>MGSSHHHHHHSSGLRNAYTERDMLQKAADETTLKNVLVMKQAWVPYPAYTDRAAWDSLMGSNKQRLIAAGEKLLDYKWQLIPATAYLEYERTGNRKIMEVPYDANRQALNTLMLAELAEGKGRFIDQLLNGAYMSCEMNSWVLSAHLPRQSSKRSLPDFREQIIDLGSGGYGALMAWVHYFFRKPFDKINPVVSLQMRKAIKERILDPYMNDDDMWWMAFNWQPGEIINNWNPWCNSNALQCFLLMENNKDRLAKAVYRSMKSVDKFINFVKSDGACEEGTSYWGHAAGKLYDYLQILSDGTGGKISLLNEPMIRRMGEYMSRSYVGNGWVVNFADASAQGGGDPLLIYRFGKAVNSNEMMHFAAYLLNGRKPYATMGNDAFRSLQSLLCCNDLAKETPKHDMPDVTWYPETEFCYMKNKNGMFVAAKGGFNNESHNHNDVGTFSLYVNTIPVILDAGVGTYTKQTFGKDRYTIWTMQSNYHNLPMINGIPQKYGQEYKATNTTCNEKKRVFSTDIAAAYPSEAKVKNWIRSYTLDDRKLTITDSYTLEEAVAPNQVNFMTWGNVTFPSQGKIQIEVKGQKVELDYPTLFKAELETIQLDDPRLSNVWGKEIYRITLKTNEKKETGNYKFVIQQIK[2x]

In bacteria, however, a different strategy employing a class of enzyme known as polysaccharide lyases (PL) is deployed. PLs selectively target glycans composed of uronic acids with a C4 hydroxyl group linked to the preceding sugar in the glycan chain. This enables PLs to operate through a β-elimination mechanism that relies on proton abstraction from the C5 carbon of the uronic acid sugar ring, resulting in double bond formation between C4 and C5 and elimination of the preceding sugar. The three characterized PL33_1 enzymes were all from Bacteroides species inhabiting the human colon: BT4410 (BtPL33HA) and BcellWH2_04512 (BcPL33HA) are hyaluronidases from Bacteroides thetaiotaomicron VPI-5482 (B. theta) and Bacteroides cellulosilyticus WH2 (B. cell), respectively, while HMPREF1181_01744 (BsPL33Heparosan) is a heparosanase from Bacteroides stercoris CC31F (B. stercoris). The enzymes are 68% identical and contain a larger N-terminal α-helical (α/α)6 toroid domain (residues 21 to 401; BtPL33HA numbering used throughout this section unless specified) and a smaller β-sheet C-terminal domain (residues 402 to 635).

Crystal structures of BtPL33HA and BcPL33HA reveal a two-domain structure. The C-terminal domain possesses an extended loop region between β-strands 5 and 6 (Leu455-Leu484: BtPL33HA, and Ile464-Leu493: BcPL33HA), forming an octahedral Zn2+ coordination site [supported by anomalous X-ray diffraction data], along with the loop region between α-helices 12 and 13 from the N-terminal domain. The two domains oppose each other in such a way that a deep, open-ended cleft is formed resembling an active site that would be compatible with an endo-processive mode of action of BtPL33HA and BcPL33HA. Analysis of the five enzymes via SEC-coupled light scattering and SAXS indicated that the three PL33_1 enzymes BtPL33HA, BcPL33HA, and BsPL33Heparosan are dimeric, while the PL33_2 enzymes ObPL33CS and ObPL33Gellan are monomeric. SAXS data indicate that the dimeric enzymes all bind as head-to-head homodimers, generating elongated envelopes. This is consistent with PISA analysis of the crystal structures of BtPL33HA and BcPL33HA which predicted a buried surface area of ~1,388 Å2 and 1,006 Å2, and a complex significance score of 0.207 and 0.290, respectively. For all five of the analyzed enzymes, AF2-generated models display a closed tunnel-like topography housing the +2 and +1 subsites. The phenol of Y470 moves within 5 to 6 Å of the +1 GlcA and N-acetyl of the −1 GlcNAc, while F475 moves within 5 Å of the +2 GlcNAc, forming the tunnel topography. This differs significantly from the wide-open cleft observed in the crystal structures of both BtPL33HA and BcPL33HA. Fitting of both the BtPL33HA and BcPL33HA crystal structures and their AF2 models to SAXS data indicated that the best fit was for the open conformation observed in the crystal structures.>[4x]MDQFIKQDETGDLIETGMNVANHFLSTPIQGTNSLSKASILPGVAPVLIGNPEQKNIQHPTASHQGSKTKGRGSGVRSIIVSPSEAGNGGTQIPEPLFAQTGQGGIVTTVYQD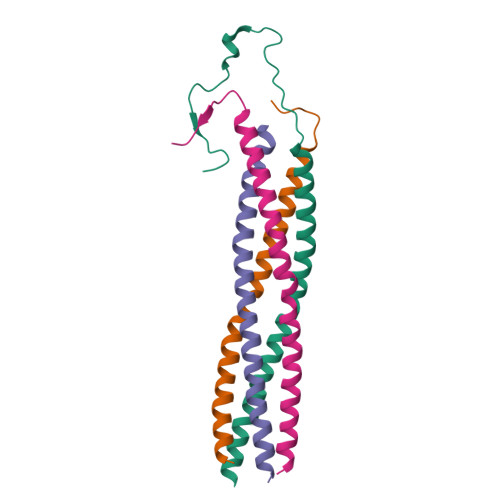PTIQPTGSYRSVELAKIGKERMINRFVEKPRTSTPVTEFKRGGPGAAAQGQTIQEEGIDGNGASAGSKERSGSLSGATLYAHLSLPQQDSTPANVGIAPQSAISANEIMDLLRGMDARLQHLEQKVDKVLAQGSMVTQIKNELSTVKTTLATIEGMMATVKIMDPGNPTGVPVDELRRSFSDHVTIVSGPGDVSFSSSEKPTLYLDELARPVSKPRPAKQTKSQPVKDLAGQKVMITKMITDCVANPQMKQAFEQRLAKASTEDALNDIKRDIIRSAI> GPGSSLCSKKDVRNFKAWFLPIMYSIICFVGLLGNGLVVLTYIYFKRLKTMTDTYLLNLAVADILFLLTLPFWAYSAAKSWVFGVHFCKLIFAIYKMSFFSGMWLLLCISIDRYVAIVQAVSAHRHRARVLLISKLSCVGIWILATVLSIPELLYSDLQRSSSEQAMRCSLITEHVEAFITIQVAQMVIGFLVPLLAMSFCYLVIISKLHALTEKTDIFESGRNGNPNKDGIKSYRIPALLKTDKGTLIAGADERRLHSSDWGDIGMVIRRSEDNGKTWGDRVTITNLRDNPKASDPSIGSPVNIDMVLVQDPETKRIFSIYDMFPEGKGIFGMSSQKEEAYKKIDGKTYQILYREGEKG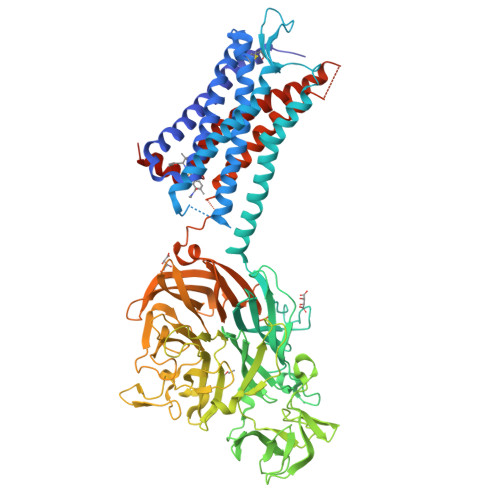AYTIRENGTVYTPDGKATDYRVVVDPVKPAYSDKGDLYKGDQLLGNIYFTTNKTSPFRIAKDSYLWMSYSDDDGKTWSAPQDITPMVKADWMKFLGVGPGTGIVLRNGPHKGRILIPVYTTNNVSHLDGSQSSRVIYSDDHGKTWHAGEAVNDNRQVDGQKIHSSTMNNRRAQNTESTVVQLNNGDVKLFMRGLTGDLQVATSKDGGVTWEKDIKRYPQVKDVYVQMSAIHTMHEGKEYIILSNAGGPKRENGMVHLARVEENGELTWLKHNPIQKGEFAYNSLQELGNGEYGILYEHTEKGQNAYTLSFRKFNWEFLSKSKGHERNKAIKVIIAVVVVFIVFQLPYNGVVLAQTVANFNITSSTCELSKQLNIAYDVTYSLACVRCCVNPFLYAFIGVKFRNDLFKLFKDLGCLSGGRLEVLFQ> DDPIGLFVMRPQDGEVTVGGSITFSARVAGASLLKPPVVKWFKGKWVDLSSKVGQHLQLHDSYDRASKVYLFELHITDAQPAF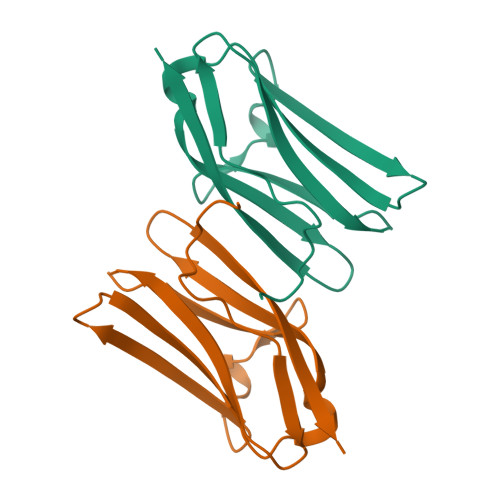TGSYRCEVSTKDKFDCSNFNLTVHE N-METHYL(5-(PYRIDIN-3-YL)FURAN-2-YL)METHANAMINE | C11 H12 N2 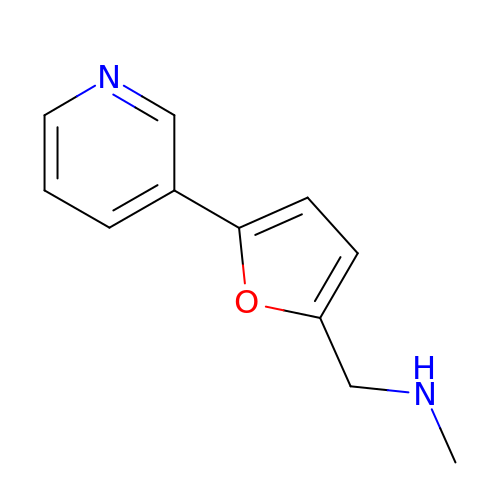O | MDGMPFRIYUFRRX-UHFFFAOYSA-N> DISKVAWAWF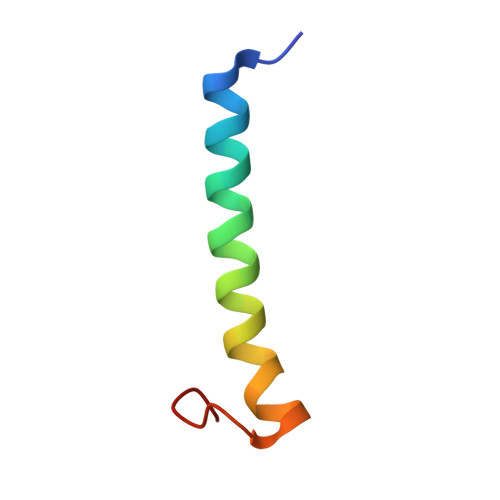GVLLAICLIGAFGNYVPKLFVKMLMFLN> MAIPKIASYQVLPLESFPTNKVD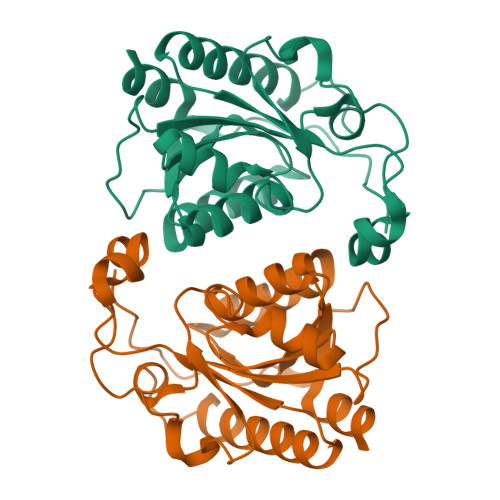WVIDPKKSVVLVHDLQAYFLNFFDKTLSPVPELLRNVNKVTESARSAGIPVVYTAQPANQDPNERALLTDFWGVGLTQDTEIVPEVSPQPEDIQYTKWRYSAFKKTPLLEWMKEEQRDQLVIVGVYGHIGILSTALDAFMLDIKPFVIGDAIADFSKEDHMNTLKYVASRSGSVKSVDEFIDSVT;> MAIPKIASYQVLPLESFPTNKVDWVIDPKKSVVLVHDLQAYFLNFFDKTLSPVPELLRNVNKVTESARSAGIPVVYTAQPANQDPNERALLTDFWGVGLTQDTEIVPEVSPQPEDIQYTKWRYSAFKKTPLLEWMKEEQRDQLVIVGVYGHIGILSTALDAFMLDIKPFVIGDAIADFSKEDHMNTLKYVASRSGSVKSVDEFISSVT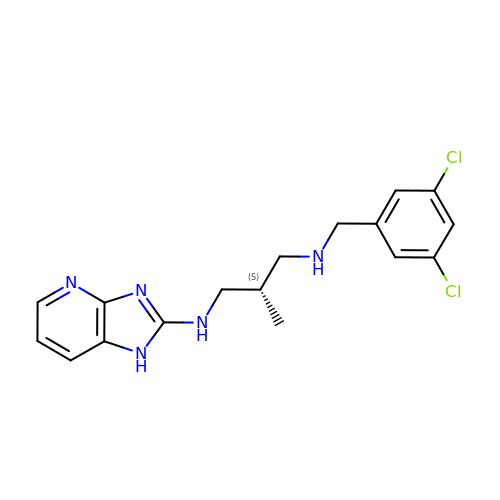(2S)-N-(3,5-dichlorobenzyl)-N'-(1H-imidazo[4,5-b]pyridin-2-yl)-2-methylpropane-1,3-diamine | C17 H19 Cl2 N5 | WHJDPLYTLYNDOF-NSHDSACASA-N>MSGTEEAILGGRDSHPAAGGGSVLCFGQCQYTAEEYQAIQKALRQRLGPEYISSRMAGGGQKVCYIEGHRVINLANEMFGYNGWAHSITQQNVDFVDLNNGKFYVGVCAFVRVQLKDGSYHEDVGYGVSEGLKSKALSLEKARKEAVTDGLKRALRSFGNALGNCILDKDYLRSLNKLPRQLPLEVDLTKAKRQDLEPSVEEARYNSCRPNMALGHPQLQQVTSPSRPSHAVIPADQDCSSRSLSSSAVESEATHQRKLRQKQLQQQFRERMEKQQVRVSTPSAEKSEAAPPAPPVTHSTPVTVSEPLLEKDFLAGVTQELIKTLEDNSEKWAVTPDAGDGVVKPSSRADPAQTSDTLALNNQMVTQNRTPHSVCHQKPQAKSGSWDLQTYSADQRTTGNWESHRKSQDMKKRKYDPS[11x]

Central to these functions, RAD52 promotes the annealing of complementary single-stranded DNA (ssDNA)8,9 and provides an alternative to BRCA2/RAD51-dependent homologous recombination repair. Instead, cryo-electron microscopy and biochemical analyses revealed that ssDNA annealing is driven by RAD52 open rings in association with replication protein-A (RPA). RPA associates with RAD52 at the site of ring opening with critical interactions occurring between the RPA-interacting domain of RAD52 and the winged helix domain of RPA2. Our studies provide structural snapshots throughout the annealing process and define the molecular mechanism of ssDNA annealing by the RAD52–RPA complex.

When visualized using cryo-EM, we found that the two species of full-length RAD52 represent open (RAD52-OR, peak 1) and closed (RAD52-CR, peak 2) ring forms. The 11-subunit closed rings exhibit features similar to the RAD52 NTD, whereas the RAD52 open rings have one or more subunits missing. The structures of RAD52-CR (2.9 Å) and RAD52-OR (3.2 Å) were determined using cryo-EM. The closed ring comprised 11 subunits as observed previously. RAD52 forms undecameric (11-subunit) ring structures, but these rings do not represent the active form of the enzyme. By contrast, the RAD52 closed rings bound to ssDNA with reduced affinity (3.3 ± 0.5 nM) comparable to that of the RAD52 NTD (3.2 ± 0.6 nM). The RAD52-ORs annealed ssDNA in reactions stimulated by RPA, whereas the RAD52-CRs exhibited a reduced ability to promote annealing that was unaffected by the presence or absence of RPA. RAD52 open rings form more stable complexes with ssDNA (40 nucleotides) and RPA compared with RAD52 closed rings, as measured in pull-down experiments, which may explain why the RAD52-CRs do not cooperate with RPA in SSA. The closed rings may be an artifact of protein overexpression.> GSMADEATRRVVSEIPVLKTNAGPRDRELWVQRLKEEYQSLIRYVENNKNADNDWFRLESNKEGTRWFGKCWYIH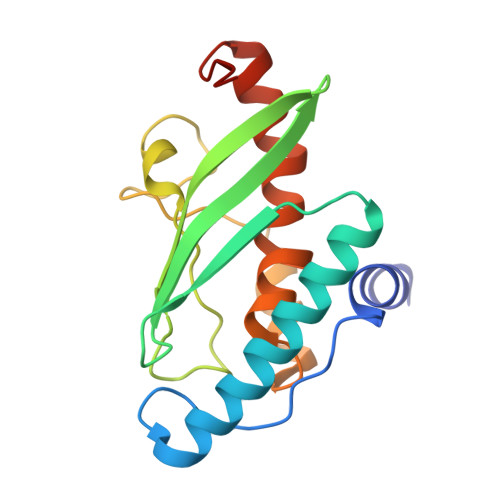DLLKYEFDIEFDIPITYPTTAPEIAVPELDGKLAKMYRGGKICLTDHFKPLWARNVPKFGLAHLMALGLGPWLAVEIPDLIQKGVIHHKEKCNQ>[6x]CSLIPDYQRPEAPVAAAYPQGQAYGQNTGAAAVPAADIGWREFFRDPQLQQLIGVALENNRDLRVAALNVEAFRAQYRIQRADLFPRIGVDGSGTRQRLP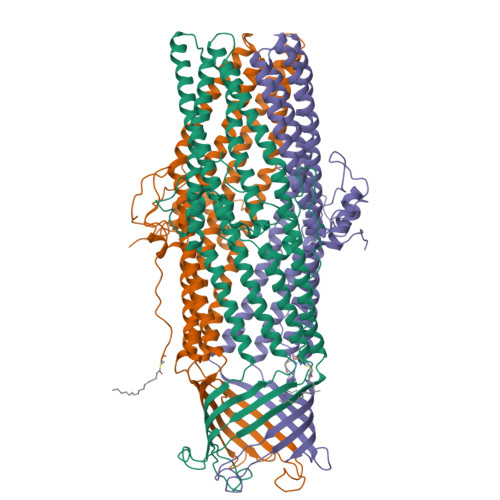GDLSTTGSPAISSQYGVTLGTTAWELDLFGRLRSLRDQALEQYLATEQAQRSAQTTLVASVATAYLTLKADQAQLQLTKDTLGTYQKSFDLTQRSYDVGVASALDLRQAQTAVEGARATLAQYTRLVAQDQNALVLLLGSGIPANLPQGLGLDQTLLTEVPAGLPSDLLQRRPDILEAEHQLMAANASIGAARAAFFPSISLTANAGTMSRQLSGLFDAGSGSWLFQPSINLPIFTAGSLRASLDYAKIQKDINVAQYEKAIQTAFQEVADGLAARGTFTEQLQAQRDLVKASDEYYQLADKRYRTGVDNYLTLLDAQRSLFTAQQQLITDRLNQLTSEVNLYKALGGGWNQQTVTQQQTAKKEDPQAHHHHHH4-(3-aminopropoxy)-8-({[4-(3-aminopropoxy)-8-({[4-(3-aminopropoxy)-8-({[4-(3-aminopropoxy)-8-nitroquinolin-2-yl]carbonyl}amino)quinolin-2-yl]carbonyl}amino)quinolin-2-yl]carbonyl}amino)quinoline-2-carboxylic 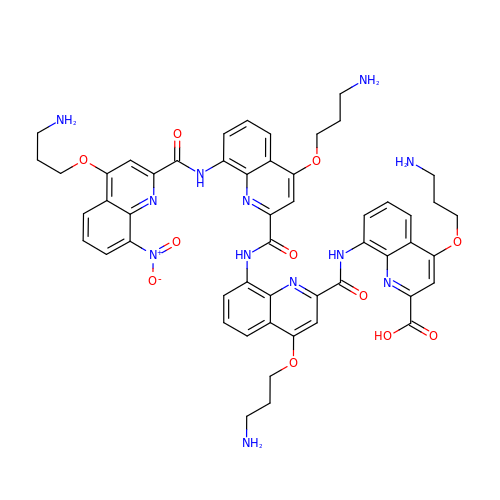acid | C52 H52 N12 O11 | PDPDTUNURBJNEI-UHFFFAOYSA-N>GEFPLQTKTDIHAVLASNGRIIYISANSKLHLGYLQGEMIGSFLKTFLHEEDQFLVESYFYNEHHLMPCTFRFIK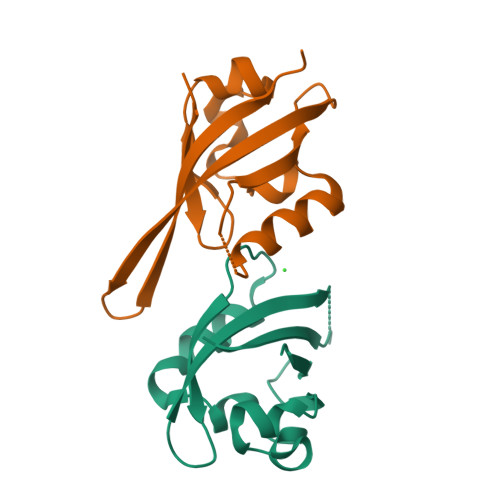KDHTIVWVEAAVEIVTTRAERTEREIILKMKVLEEE[4x]>GSHMASLTEIEHLVQSVCKSYRETCQLRLEDLLRQRSNIFSREEVTGYQRKSMWEMWERCAHHLTEAIQYVVEFAKRLSGFMELCQNDQIVLLKAGAMEVVLVRMCRAYNADNRTVFFEGKYGGMELFRALGCSELISSIFDFSHSLSALHFSEDEIALYTALVLINAHRPGLQEKRKV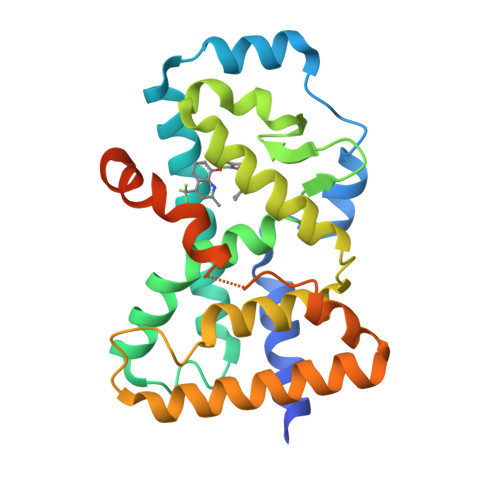EQLQYNLELAFHHHLCKTHRQSILAKLPPKGKLRSLCSQHVERLQIFQHLHPIVVQAAFPPLYKELFS[2x]3-[5-({5-[(AMINOCARBONYL)AMINO]-2-OXO-2H-INDOL-3-YL}METHYL)-1H-PYRROL-3-YL]-N-(2-PIPERIDIN-1-YLETHYL)BENZAMIDE | C28 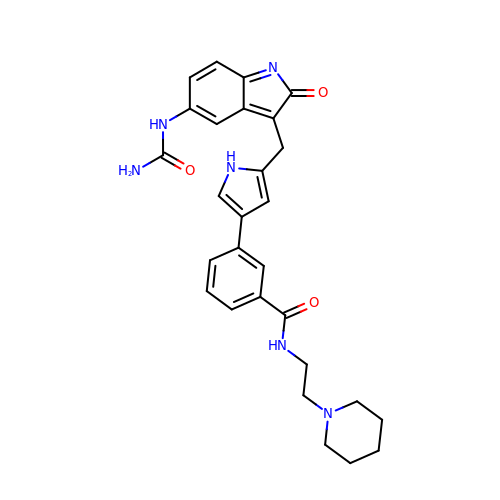H30 N6 O3 | PWZOBKJHPWISGC-UHFFFAOYSA-N4-{2-[(3-NITROBENZOYL)AMINO]PHENOXY}PHTHALIC 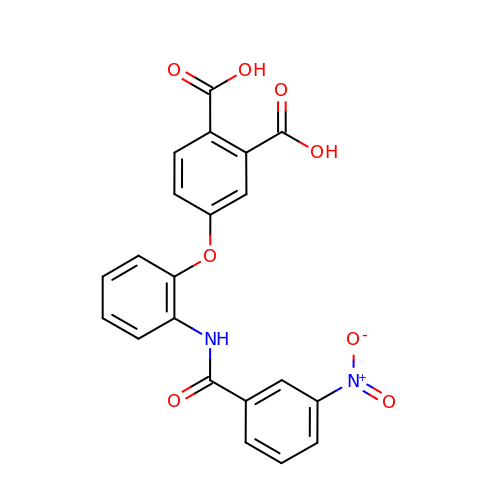ACID | C21 H14 N2 O8 | NAQUAVBNIYTIIS-UHFFFAOYSA-N>GSMHLRPIATPYPVKEWLQPKRYKAHLMGTTYVYDFPELFRQASSSQWKNFSADVKLTDDFFISNELIEDENGELTEVEREPGANAIGMVAFKITVKTPEYPRGRQFVVVANDITFKIGSFGPQEDEFFNKVTEYARKRGIPRIYLAANSGARIGMAEEIVPLFQVAWNDAANPDKGFQYLYLTSEGMETLKKFDKENSVLTERTVINGEERFVIKTIIGSEDGLGVECLRGSGLIAGATSRAYHDIFTITLVTCRSVGIGAYLVRLGQRAIQVEGQPIILTGAPAINKMLGREVYTSNLQLGGTQIMYNNGVSHLTAVDDLAGVEKIVEWMSYVPAKRNMPVPILETKDTWDRPVDFTPTNDETYDVRWMIEGRETESGFEYGLFDKGSFFETLSGWAKGVVVGRARLGGIPLGVIGVETRTVENLIPADPANPNSAETLIQEPGQVWHPNSAFKTAQAINDFNNGEQLPMMILANWRGFSGGQRDMFNEVLKYGSFIVDALVDYKQPIIIYIPPTGELRGGSWVVVDPTINADQMEMYADVNARAGVLEPQGMVGIKFRREKLLDTMNRLDDKYRELRSQLSNKSLAPEVHQQISKQLADRERELLPIYGQISLQFADLHDRSSRMVAKGVISKELEWTEARRFFFWRLRRRLNEEYLIKRLSHQVGEASRLEKIARIRSW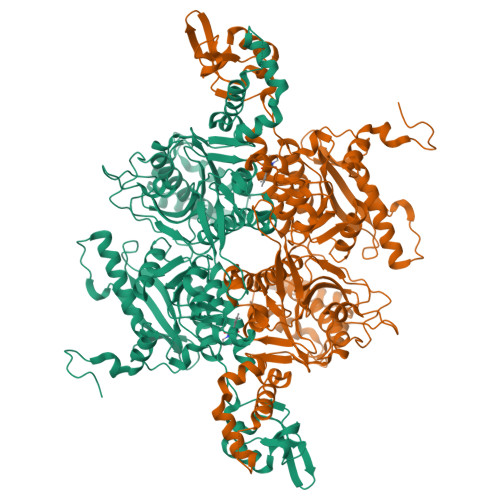YPASVDHEDDRQVATWIEENYKTLDDKLKGLKLESFAQDLAKKIRSDHDNAIDGLSEVIKMLSTDDKEKLLKTLKHHHHHH[3x]> RSVPSSTILIPVVVHVVYNNSAQNISDAQIISQIQVLNEDFRRMNADQANTPSAFANLAGNANIEFKLARRDPNGNTTNGITRTSTSTETFSMEMDNVKFSNLGGNNAWNTRRYLNIWVCNLGDDLLGYAQFPFE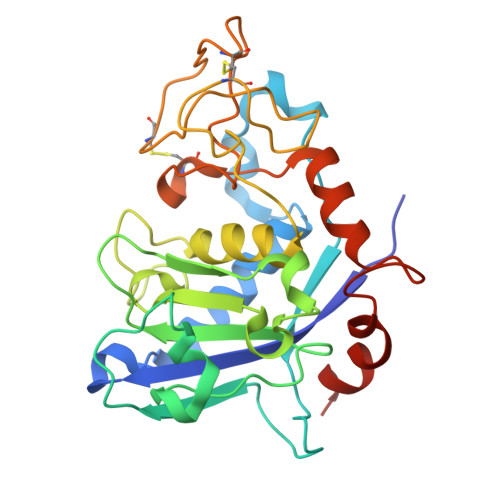FQTKPNTDGVVIHYKHFGRDGSAESPYDKGRTATHEVGHWLDLRHIWGDDGGSCSGTDNIADTPNQGGYNEGCPSFPKTDHCTNTSPGVMFMNYMDYTYDACMNLFTKGQVERMRSLFDTQTGIRREMQIYANELTNPLSFS(S)-{4-chloro-2-methoxy-3-[4-(methylsulfonyl)phenyl]quinolin-6-yl}(1-methyl-1H-imidazol-5-yl)[6-(trifluoromethyl)pyridin-3-yl]methanol 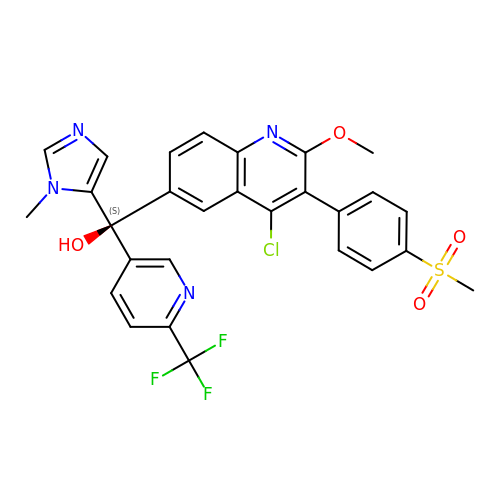| C28 H22 Cl F3 N4 O4 S | GBSZBTDJEFDZLG-MHZLTWQESA-N>MGDLSCPEGLEELLSAPPPDLGAQRRHGWNPKDCSENIEVKEGGLYFERRPVAQSTDGARGKRGYSRGLHAWEISWPLEQRGTHAVVGVATALAPLQTDHYAALLGSNSESWGWDIGRGKLYHQSKGPGAPQYPAGTQGEQLEVPERLLVVLDMEEGTLGYAIGGTYLGPAFRGLK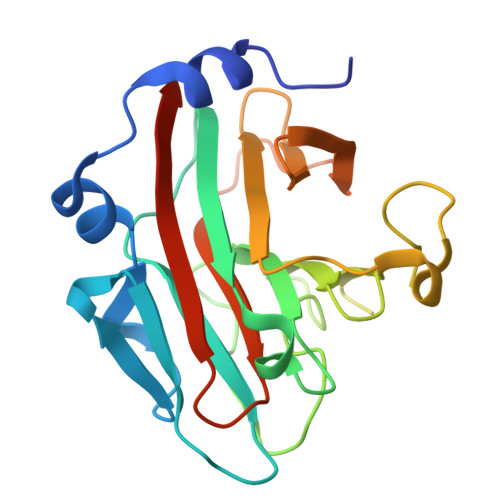GRTLYPAVSAVWGQCQVRIRYLGERGSHHHHHH[2x]4-[(3,4-dihydroisoquinolin-2(1H)-yl)methyl]phenol | C16 H17 N O | 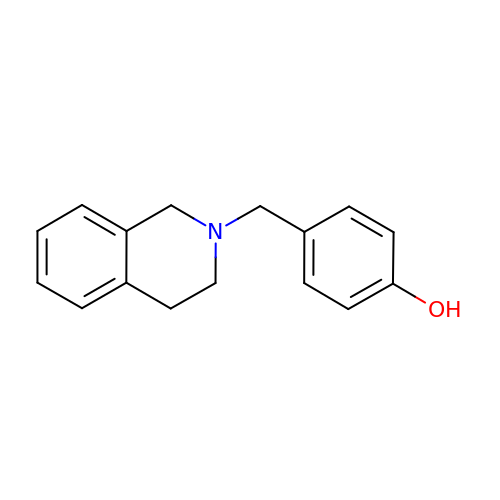INQGOEXXFRCTEG-UHFFFAOYSA-N> NSLDRAQAAKNKGNKYFKAGKYEQAIQCYTEAISLCPTEKNVDLSTFYQNRAAAFEQLQKWKEVAQDCTKAVELNPKYVKALFRRAKAHEKLDNKKECLEDVTAVCILEGFQNQQSMLLADKVLKLLGKEKAKEKYKNREPLMPSPQFIKSYFSSFTDDIISQPMLK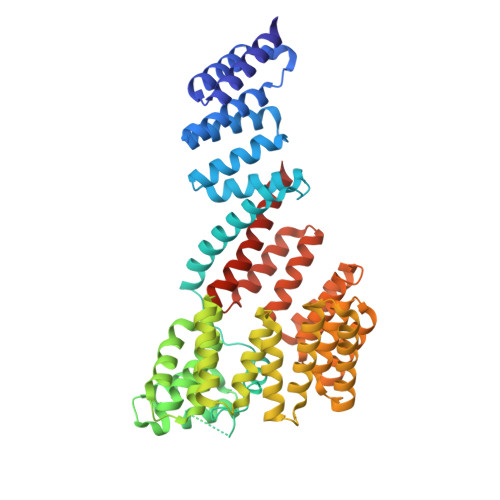GEKSDEDKDKEGEALEVKENSGYLKAKQYMEEENYDKIISECSKEIDAEGKYMAEALLLRATFYLLIGNANAAKPDLDKVISLKEANVKLRANALIKRGSMYMQQQQPLLSTQDFNMAADIDPQNADVYHHRGQLKILLDQVEEAVADFDECIRLRPESALAQAQKCFALYRQAYTGNNSSQIQAAMKGFEEVIKKFPRCAEGYALYAQALTDQQQFGKADEMYDKCIDLEPDNATTYVHKGLLQLQWKQDLDRGLELISKAIEIDNKCDFAYETMGTIEVQRGNMEKAIDMFNKAINLAKSEMEMAHLYSLCDAAHAQTEVAKKYGLKPPTL> MSLRRGIYHIENAGVPSAIDLKDGSSSDGTPIVGWQFTPDTINWHQLWLAEPIPNVADTFTLCNLFSGTYMDLYNGSSEAGTAVNGWQGTAFTTNPHQLWTIKKSSDGTSYKIQNYGSKTFVDLVNGDSSDGAKIAGWTGTWDEGNPHQKWYFNRMSVSSAEAQAAIARNPHIHGTYRGYILDGEYLVLPNATFTQIWKDSGLPGSKWRE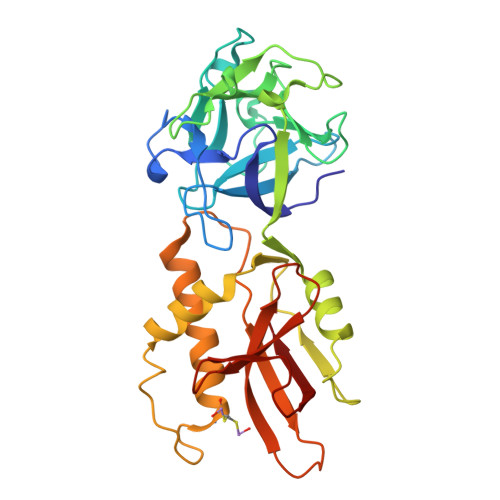QIYDCDDFAIAMKAAVGKWGADSWKANGFAIFCGVMLGVNKAGDAAAAYNFTLTKDHADIVFFEPQNGGYLNDIGYDSYMAFY>[2x]MKPKVLITRAIPENGIELLREHFEVEVWEHEHE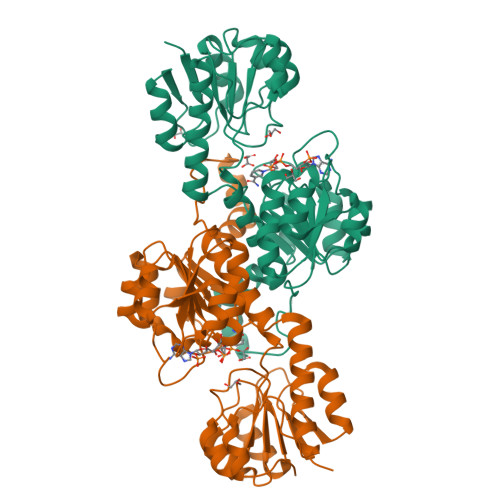IPREVLLEKVKDVDALVTMLSEKIDREVFDAAPRLRIVANYAVGYDNIDIEEATKRGIYVTNTPDVLTDATADLAWALLLAAARHVVKGDKFVRSGEWKRRGIAWHPKMFLGYDVYGKTIGIVGFGRIGQAIAKRAKGFGMRILYTARSRKPEAEKELGAEFKPLEELLRESDFVVLAVPLTKETYHMINEERLRLMKPTAVLVNVARGKVVDTKALIRALKEGWIAAAGLDVFEEEPYYDEELFALDNVVLTPHIGSATFGAREGMAELVAKNLIAFKNGEVPPTLVNREVLKVRRPGF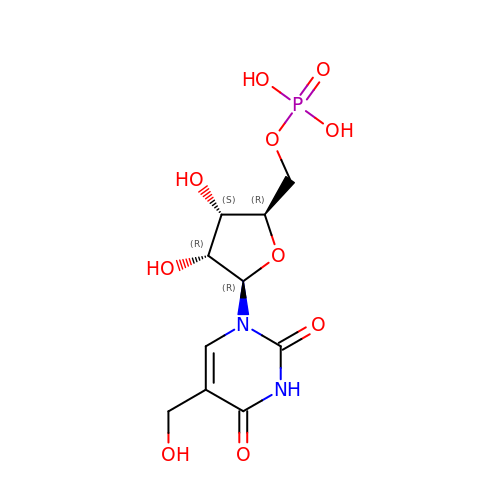5-(hydroxymethyl)uridine 5'-(dihydrogen phosphate) | C10 H15 N2 O10 P | WQCABYUOJVUOEC-JXOAFFINSA-N>MHHHHHHSSGRENLYFQGMTATTRGSPVGGNDNQGQAPDGQSQPPLQQNQTSSPDSSNENSPATPPDEQGQGDAPPQLEDEEPAFPHTDLAKLDDMINRPRWVVPVLPKGELEVLLEAAIDLSKKGLDVKSEACQRFFRDGLTISFTKILTDEAVSGWKFEIHRCIINNTHRLVELCVAKLSQDWFPLLELLAMALNPHCKFHIYNGTRPCESVSSSVQLPEDELFARSPDPRSPKGWLVDLLNKFGTLNGFQILHDRFINGSALNVQIIAALIKPFGQCYEFLTLHTVKKYFLPIIEMVPQFLENLTDEELKKEAKNEAKNDALSMIIKSLKNLASRVPGQEETVKNLEIFRLKMILRLLQISSFNGKMNALNEVNKVISSVSYYTHRHGNPEEEEWLTAERMAEWIQQNNILSIVLRDSLHQPQYVEKLEKILRFVIKEKALTLQDLDNIWAAQAGKHEAIVKNVHDLLAKLAWDFSPEQLDHLFDCFKASWTNASKKQREKLLELIRRLAEDDKDGVMAHKVLNLLWNLAHSDDVPVDIMDLALSAHIKILDYSCSQDRDTQKIQWIDRFIEELRTNDKWVIPALKQIREICSLFGEAPQNLSQTQRSPHVFYRHDLINQLQHNHALVTLVAENLATYMESMRLYARDHEDYDPQTVRLGSRYSHVQEVQERLNFLRFLLKDGQLWLCAPQAKQIWKCLAENAVYLCDREACFKWYSKLMGDEPDLDPDINKDFFESNVLQLDPSLLTENGMKCFERFFKAVNCREGKLVAKRRAYMMDDLELIGLDYLWRVVIQSNDDIASRAIDLLKEIYTNLGPRLQVNQVVIHEDFIQSCFDRLKASYDTLCVLDGDKDSVNCARQEAVRMVRVLTVLREYINECDSDYHEERTILPMSRAFRGKHLSFVVRFPNQGRQVDDLEVWSHTNDTIGSVRRCILNRIKANVAHTKIELFVGGELIDPADDRKLIGQLNLKDKSLITAKLTQISSNMPSSPDSSSDSSTGSPGNHGNHYSDGPNPEVESCLPGVIMSLHPRYISFLWQVADLGSSLNMPPLRDGARVLMKLMPPDSTTIEKLRAICLDHAKLGESSLSPSLDSLFFGPSASQVLYLTEVVYALLMPAGAPLADDSSDFQFHFLKSGGLPLVLSMLTRNNFLPNADMETRRGAYLNALKIAKLLLTAIGYGHVRAVAEACQPGVEGVNPMTQINQVTHDQAVVLQSALQSIPNPSSECMLRNVSVRLAQQISDEASRYMPDICVIRAIQKIIWASGCGSLQLVFSPNEEITKIYEKTNAGNEPDLEDEQVCCEALEVMTLCFALIPTALDALSKEKAWQTFIIDLLLHCHSKTVRQVAQEQFFLMCTRCCMGHRPLLFFITLLFTVLGSTARERAKHSGDYFTLLRHLLNYAYNSNINVPNAEVLLNNEIDWLKRIRDDVKRTGETGIEETILEGHLGVTKELLAFQTSEKKFHIGCEKGGANLIKELIDDFIFPASNVYLQYMRNGELPAEQAIPVCGSPPTINAGFELLVALAVGCVRNLKQIVDSLTEMYYIGTAITTCEALTEWEYLPPVGPRPPKGFVGLKNAGATCYMNSVIQQLYMIPSIRNGILAIEGTGSDVDDDMSGDEKQDNESNVDPRDDVFGYPQQFEDKPALSKTEDRKEYNIGVLRHLQVIFGHLAASRLQYYVPRGFWKQFRLWGEPVNLREQHDALEFFNSLVDSLDEALKALGHPAMLSKVLGGSFADQKICQGCPHRYECEESFTTLNVDIRNHQNLLDSLEQYVKGDLLEGANAYHCEKCNKKVDTVKRLLIKKLPPVLAIQLKRFDYDWERECAIKFNDYFEFPRELDMEPYTVAGVAKLEGDNVNPESQLIQQSEQSESETAGSTKYRLVGVLVHSGQASGGHYYSYIIQRNGGDGERNRWYKFDDGDVTECKMDDDEEMKNQCFGGEYMGEVFDHMMKRMSYRRQKRWWNAYILFYERMDTIDQDDELIRYISELAITTRPHQIIMPSAIERSVRKQNVQFMHNRMQYSMEYFQFMKKLLTCNGVYLNPPPGQDHLLPEAEEITMISIQLAARFLFTTGFHTKKVVRGSASDWYDALCILLRHSKNVRFWFAHNVLFNVSNRFSEYLLECPSAEVRGAFAKLIVFIAHFSLQDGPCPSPFASPGPSSQAYDNLSLSDHLLRAVLNLLRREVSEHGRHLQQYFNLFVMYANLGVAEKTQLLKLSVPATFMLVSLDEGPGPPIKYQYAELGKLYSVVSQLIRCCNVSSRMQSSINGNPPLPNPFGDPNLSQPIMPIQQNVADILFVRTSYVKKIIEDCSNSEETVKLLRFCCWENPQFSSTVLSELLWQVAYSYTYELRPYLDLLLQILLIEDSWQTHRIHNALKGIPDDRDGLFDTIQRSKNHYQKRAYQCIKCMVALFSNCPVAYQILQGNGDLKRKWTWAVEWLGDELERRPYTGNPQYTYNNWSPPVQSNETSNGYFLE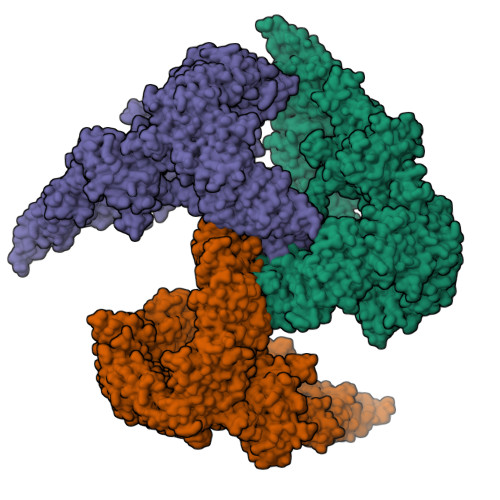RSHSARMTLAKACELCPEEEPDDQDAPDEHESPPPEDAPLYPHSPGSQYQQNNHVHGQPYTGPAAHHMNNPQRTGQRAQENYEGSEEVSPPQTKDQDYKDDDK[3x]> EYEERES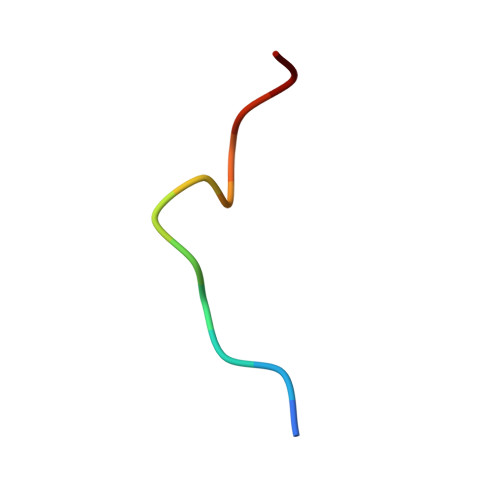EFDIE> ARPTFHITVGDPHKVGDLATSHIVYSVR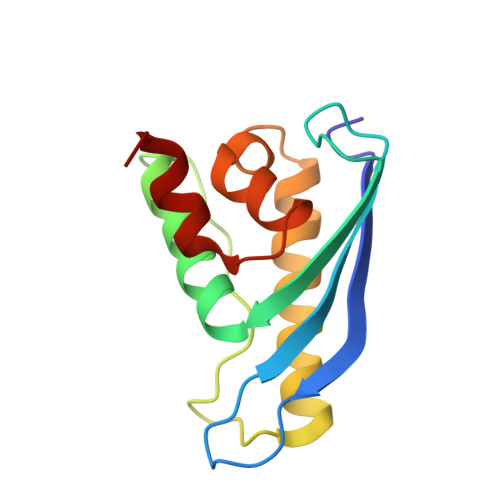TKTTSKAYKQPEFEVKRRYRDFLWLYNTLHSNNPGVVVPPPPEKQAVGRFESNFVESRRAALEKMLNKIAAHPTLQLDADLKLFLESESFNIDVKHKERKE> MDDDVKSWIMNEFSGSTDGKGGDDAKAQQRARGRKGHSAAMDAEKLAASSLFTWDFDALDKSDEDLTAVCVRVFQELHVIEQFNIDEKKLRKWLQKVRTQYNKNPFHNWRHAVMVLHTTYLLLTSVATEFITEVELLAMLIAALSHDLDHNGLTNAFHINSRSELALVYNDQSVLENHHSHLAFEILLEKGCNVVENLDE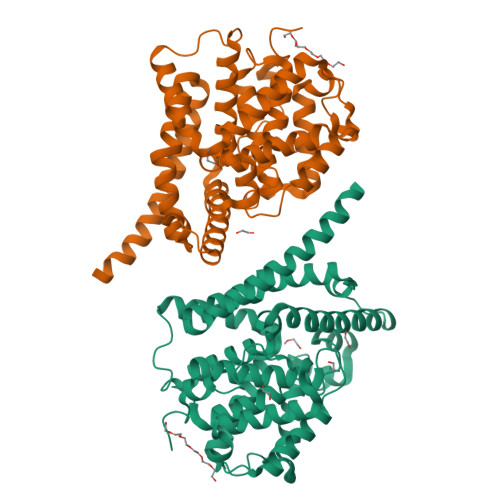DEFKRLRAVIINCILNTDMATHHTKLSKMEEVNRLGGFINLAENNDQRLFVLAVLLHTADLHNPIKPFESNKRWSARLQKEFNNQVELEAKMNLPSLPFMRGNDEESLAKGEIGFINFVVKPWHQQLSQAFPKLDFLLDTIDANLAEWKAIAESYRQMQENLYFQ Inherited missense mutations in the myocilin (MYOC) gene, within its olfactomedin (OLF) domain, constitute the strongest genetic link to primary open-angle glaucoma via a toxic gain of function, and thus MYOC is an attractive precision-medicine target. Myocilin has no known function, and there is no glaucoma phenotype in Myoc knockout mice or in individuals with a homozygous N-terminal truncation mutation or hemizygous deletion of MYOC, but rare non-synonymous coding mutations lead to toxic intracellular sequestration of misfolded myocilin. However, not all mutations in MYOC cause glaucoma, and common variants are expected to be neutral polymorphisms. Among the common features associated with pathogenic myocilin misfolding, we demonstrate that a single metric, OLF thermal stability, can robustly segregate benign from early-onset disease variants.

At the outset of our study, five variants could be confidently predicted as benign polymorphisms: T293K, T353I, K398R, A445V and K500R. These mutations are all found on the protein surface and well documented in the literature. Three of these variants harbor conservative substitutions (Lys to Arg, Ala to Val). Modestly lower levels than WT were detected for T293K, E352K, K398R, N420Y and A427T. Structural integrity was further confirmed by high-resolution crystal structures, which were solved for 11 OLF variants. No gross changes from WT OLF were detected for the structures of T293K, R296H, L303I, V329M, S331L, E352K, T353I, K398R, A445V, V449I or K500R, indicating that these mutations are accommodated within the native five-bladed β-propeller fold and do not perturb the dinuclear calcium-containing site.

> LKESPSGYLRSGEGDTGCGELVWVGEPLTLRTAETITGKYGVWMRDPKPTYPYTQETTWRIDTVGTDVRQVFEYDLISQFMQGYPSKVHILPRPLESTGAVVYSGSLYFQGAESRTVIRYELNTETVKAEKEIPGAGYHGQFPYSWGGYTDIDLAVDEAGLWVIYSTDEARGAIVLSKLNPENLELEQTWETNIRKQSVANAFIICGTLYTVSSYTSADATVNFAYDTGTGISKTLTIPFKNRYKYSSMIDYNPLEKKLFAWDNLNMVTYDIKLSKM> GGLTQRVADGTVSATKSLFYRQIKTLHLDIRAREAINTSAAGIPLSVVVRIYQLKDNRSFDSADYQALFTGDNEILAGDIIAQKDVWLQPGGSVAVDMPLDDAAKFTGVAAMFLEPDQKKNTWRVVLGRDELEPDTPRLIEVSGNTLTLLPVKDK

Among the six secretion systems identified in Gram negative bacteria, the recently identified Type VI secretion system (T6SS) is composed of 13 core components which form a trans-envelope apparatus. We report here the crystal structure of the TssJ protein of the enteroaggregative Escherichia coli Sci1 T6SS which likely constitute a prototype for all TssJ-like proteins. We reported here the crystal structure of the TssJ lipoprotein, a critical core-component of Type VI secretion systems, and its interaction with TssM. TssJ is a β-sandwich resembling transthyretin with two additional elements: a protruding loop and a small helical domain.

The structure was solved from 2.0 Å resolution SIRAS (single isomorphous replacement with anomalous scattering) maps calculated using CsI as phasing agents, and the resolution limit was extended to 1.35 Å with the native data set. The polypeptide chain could be traced from residue Ile23 to Pro151. The segment 1-22 anchoring the protein to the membrane via Cys1 and its phospholipid thioester as well as the last four residues were not ordered in the crystal. A unique TssJ molecule is contained in the asymmetric unit, and the PISA server did not identify any sufficient interactions between TssJ molecules related by crystallographic symmetry. TssJ has the topology of a β-sandwich formed by two four-stranded β-sheets. The other face of β-sheet 2 one is covered in part by three short helices (h1-3) occurring between β-strands 2 and 3. Noteworthy, TssJ helical domain (residues 57-71) is absent in transthyretin, 5-hydroxy-isourate hydrolase and ExsB, but a single helix is located on the same face, between strands 4 and 5 of transthyretin. The extended loop (residues 38-45) between stands 1 and 2, forming a protruding extension, is also absent in the three proteins. A group of aromatic residues, Tyr65, Phe113 and Trp123 form also a structurally important hydrophobic cluster stabilizing the α-helical domain against the β-sandwich core. Coupled to the observation that TssJ-ΔL1-2 was correctly folded, we concluded that the L1-2 loop of TssJ is a critical determinant for the TssJ-TssM interaction. Collectively, the data from the in vivo and in vitro experiments demonstrate the existence of a 1∶1 stoichiometry complex between the C-terminal periplasmic domain of TssM and the TssJ lipoprotein, with a Kd of 2-4 µM.The structure of IDE is atypical with a very large catalytic chamber, called ‘crypt', formed by two joining N- and C-terminal domains. The zinc ion is located in the N-terminal domain, but key residues forming the hydrolytic site are located in both domains, resulting in constitution of the catalytic site only in the closed state. IDE has two substrate binding sites, one at the catalytic cleft and the other at the exosite that is distal away from the catalytic cleft. All of these results are consistent with the recognized role of IDE as major protease acting in the degradation of insulin and Aβ.

To substantiate our understanding of SAR, we used X-ray crystallography to determine the structure of compound 1-bound hIDE and examine the binding mode of compound 1. hIDE consists of two 50 kDa homologous N- and C-terminal domains (IDE-N and IDE-C). Compound 1 forms close contact with the catalytic site formed by both IDE-N and IDE-C of IDE. The hydroxamate tightly chelates the zinc ion at IDE-N. The fluorinated group of BDM44768 also forms a π-bond with Phe820 at IDE-C. In addition, the triazole interacts with the positively charged guanidinium of Arg824 at IDE-C. This is consistent with the high affinity of triazole for cations. Interestingly, the naphthyl side chain has some conformational freedom within a hydrophobic pocket formed in the C-terminal domain of the catalytic site. The relative freedom of the naphthyl chain in the binding pocket is consistent with limited loss of potency observed when inversing the chiral centre of 1 and explains the discontinuous electron density. The hydrophobic contacts of the naphthyl group with F820 and F834 residues are also consistent with the observed reduction in affinity when it is replaced by the phenyl group. The F-atom in compound 1 forms key hydrogen bonds with S816 and E817 but the methyl group in compound 10 does not. The 1, 4-triazole moiety allows compound 1 to complement well with the catalytic pocket of IDE, whereas 1,5-triazole makes compound 16 more compact (distance from the branching β carbon to F of compound 16 is ∼1 Å less than that of compound 1) (9.2 Å versus 10.1 Å). As it binds to the catalytic site formed by IDE-N and IDE-C, compound 1 appears to inhibit IDE by keeping the enzyme in a closed, inhibited conformation. The closed conformation is observed in the co-crystal structure with 1 and its existence in solution is strongly suggested by the SAXS experiment.

>MHHHHHHAAGIPMNNPAIKRIGNHITKSPEDKREYRGLELANGIKVLLISDPTTDKSSAALDVHIGSLSDPPNIAGLSHFLQHMLFLGTKKYPKENEYSQFLSEHAGSSNAFTSGEHTNYYFDVSHEHLEGALDRFAQFFLSPLFDESAKDREVNAVDSEHEKNVMNDAWRLFQLEKATGNPKHPFSKFGTGNKYTLETRPNQEGIDVRQELLKFHSAYYSSNLMAVVVLGRESLDDLTNLVVKLFSEVENKNVPLPEFPEHPFQEEHLKQLYKIVPIKDIRNLYVTFPIPDLQKYYKSNPGHYLGHLIGHEGPGSLLSELKSKGWVNTLVGGQKEGARGFMFFIINVDLTEEGLLHVEDIILHMFQYIQKLRAEGPQEWVFQELKDLNAVAFRFKDKERPRGYTSKIAGILHYYPLEEVLTAEYLLEEFRPDLIEMVLDKLRPENVRVAIVSKSFEGKTDRTEEWYGTQYKQEAIPDEVIKKWQNADLNGKFKLPTKNEFIPTNFEILPLEKEATPYPALIKDTAMSKLWFKQDDKFFLPKANLNFEFFSPFAYVDPLHSNMAYLYLELLKDSLNEYAYAAELAGLSYDLQNTIYGMYLSVKGYNDKQPILLKKIIEKMATFEIDEKRFEIIKEAYMRSLNNFRAEQPHQHAMYYLRLLMTEVAWTKDELKEALDDVTLPRLKAFIPQLLSRLHIEALLHGNITKQAALGIMQMVEDTLIEHAHTKPLLPSQLVRYREVQLPDRGWFVYQQRNEVHNNSGIEIYYQTDMQSTSENMFLELFAQIISEPAFNTLRTKEQLGYIVFSGPRRANGIQGLRFIIQSEKPPHYLESRVEAFLITMEKSIEDMTEEAFQKHIQALAIRRLDKPKKLSAESAKYWGEIISQQYNFDRDNTEVAYLKTLTKEDIIKFYKEMLAVDAPRRHKVSVHVLAREMDSNPVVGEFPAQNDINLSQAPALPQPEVIQNMTEFKRGLPLFPLVKPHINFMAAKL[2x]>MAEAASCARKGTKYAEGTQPFTVLIEGNIGSGKTTYLNHFEKYKNDICLLTEPVEKWRNVNGVDLLELMYKDPKKWAMPFQSYVTLTMLQSHTAPTNKKLKIMERSIFSARYCFVENMRRNGSLEQGMYNTLEEWYKFIEESIHVQADLIIYLRTSPEVAYERIRQRARSEESCVPLKYLQELHELHE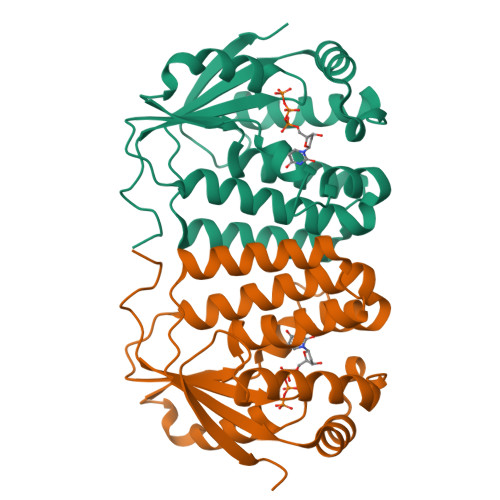DWLIHQRRPQSCKVLVLDADLNLENIGTEYQRSESSIFDAIS[4x]5-azanyl-3-[1-[[(2~{R})-1-methylpiperidin-2-yl]methyl]indol-6-yl]-1~{H}-pyrazole-4-carbonitrile | C19 H22 N6 | 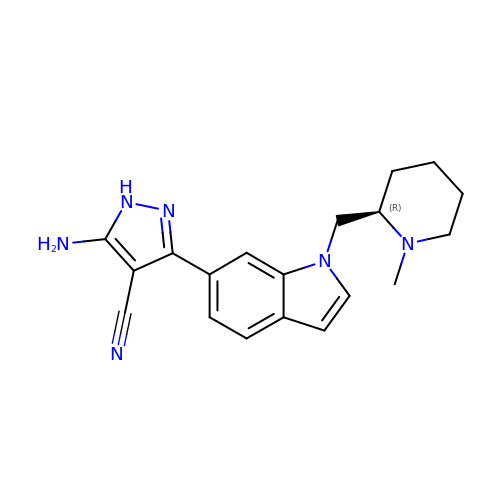SXMWJVDDIHQQEA-OAHLLOKOSA-N> G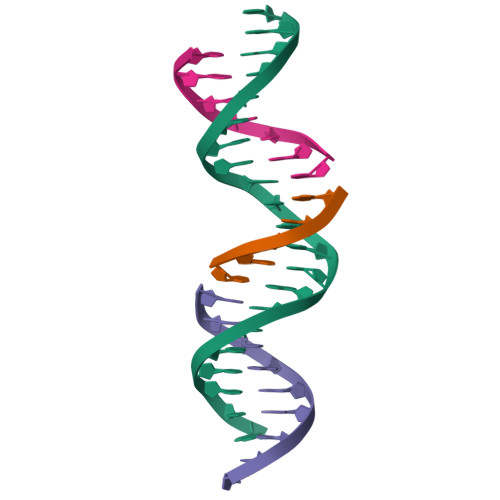AGCAGACGTGACAGCACTCA;> TGTCA;> TCTGAGTGC;> CGTCTGC> MSALPEEVNRTLLQIVQAFASPDNQIRSVAEKALSEEWITENNIEYLLTFLAEQAAFSQDTTVAALSAVLFRKLALKAPITHIRKEVLAQIRSSLLKGFLSERADSIRHKLSDAIAECVQDDLPAWPELLQALIESLKSGNPNFRESSFRILTTVPYLITAVDINSILPIFQSGFTDASDNVKIAAVTAFVGYFKQLPKSEWSKLGILLPSLLNSLPRFLDDGKDDALASVFESLIELVELAPKLFKDMFDQIIQFTDMVIKNKDLEPPARTTALELLTVFSENAPQMCKSNQNYGQTLVMVTLIMMTEVSIDDDDAAEWIESDDTDDEEEVTYDHARQALDRVALKLGGEYLAAPLFQYLQQMITSTEWRERFAAMMALSSAAEGCADVLIGEIPKILDMVIPLINDPHPRVQYGCCNVLGQISTDFSPFIQRTAHDRILPALISKLTSECTSRVQTHAAAALVNFSEFASKDILEPYLDSLLTNLLVLLQSNKLYVQEQALTTIAFIAEAAKNKFIKYYDTLMPLLLNVLKVNNKDNSVLKGKCMECATLIGFAVGKEKFHEHSQELISILVALQNSDIDEDDALRSYLEQSWSRICRILGDDFVPLLPIVIPPLLITAKATQDVGLIEEEEAANFQQYPDWDVVQVQGKHIAIHTSVLDDKVSAMELLQSYATLLRGQFAVYVKEVMEEIALPSLDFYLHDGVRAAGATLIPILLSCLLAATGTQNEELVLLWHKASSKLIGGLMSEPMPEITQVYHNSLVNGIKVMGDNCLSEDQLAAFTKGVSANLTDTYERMQDRHGDGDEYNENIDEEEDFTDEDLLDEINKSIAAVLKTTNGHYLKNLENIWPMINTFLLDNEPILVIFALVVIGDLIQYGGEQTASMKNAFIPKVTECLISPDARIR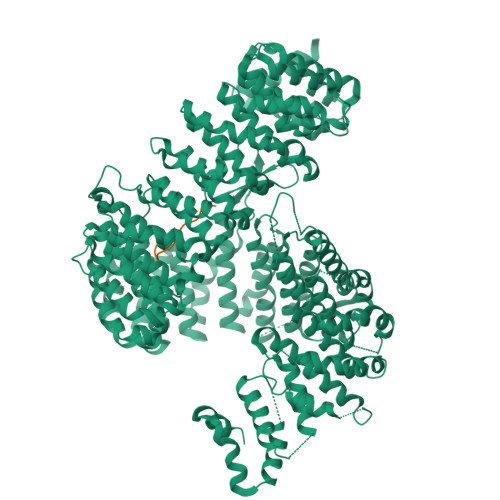QAASYIIGVCAQYAPSTYADVCIPTLDTLVQIVDFPGSKLEENRSSTENASAAIAKILYAYNSNIPNVDTYTANWFKTLPTITDKEAASFNYQFLSQLIENNSPIVCAQSNISAVVDSVIQALNERSLTEREGQTVISSVKKLLGFLPSSDAMAIFNRYPADIMEKVHKWFA;> SANKVTKNKSNSSPYLNKRRGKPGPDS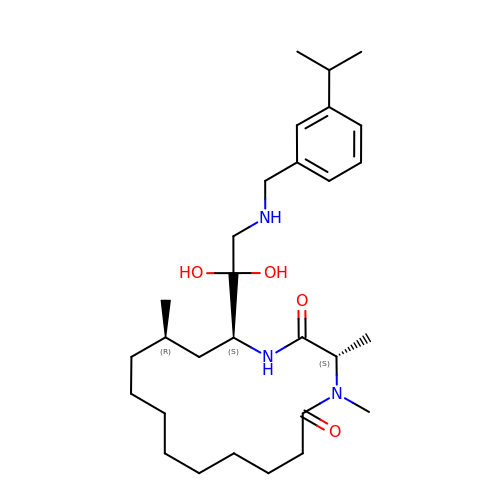(3S,14R,16S)-16-[1,1-dihydroxy-2-({[3-(propan-2-yl)phenyl]methyl}amino)ethyl]-3,4,14-trimethyl-1,4-diazacyclohexadecane-2,5-dione | C29 H49 N3 O4 | PVWMLHVFMZYBAR-UMFSSWHCSA-N> MEDKGKTFFGQPLGLSTLFMTEMWERFSYYGMRAILLYYMWFLISTGDLHITRATAASIMAIYASMVYLSG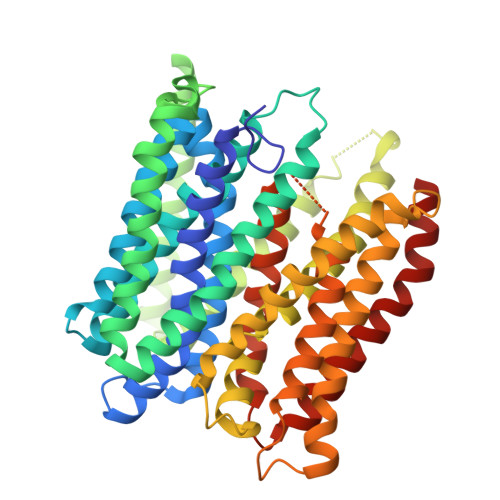TIGGFVADRIIGARPAVFWGGVLIMLGHIVLALPFGASALFGSIILIIIGTGFLKPNVSTLVGTLYDEHDRRRDAGFSIFVFGINLGAFIAPLIVGAAQEAAGYHVAFSLAAIGMFIGLLVYYFGGKKTLDPHYLRPTDPLAPEEVKPLLVKVSLAVAGFIAIIVVMNLVGWNSLPAYINLLTIVAIAIPVFYFAWMISSVKVTSTEHLRVVSYIPLFIAAVLFWAIEEQGSVVLATFAAERVDSSWFPVSWFQSLNPLFIMLYTPFFAWLWTAWKKNQPSSPTKFAVGLMFAGLSFLLMAIPGALYGTSGKVSPLWLVGSWALVILGEMLISPVGLSVTTKLAPKAFNSQMMSMWFLSSSVGSALNAQLVTLYNAKSEVAYFSYFGLGSVVLGIVLVFLSKRIQGL4-[3-cyano-2-oxo-7-(1H-pyrazol-4-yl)-5,6-dihydro-1H-benzo[h]quinolin-4-yl]benzoic 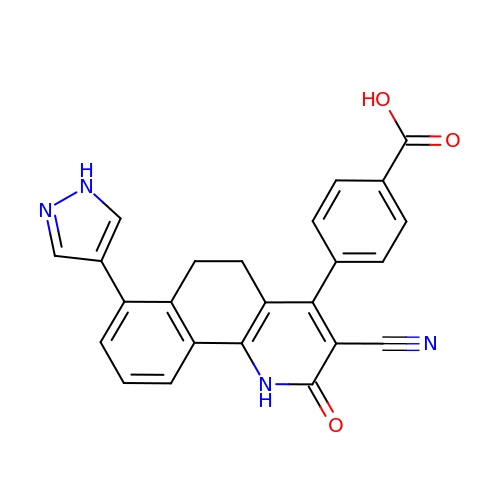acid | C24 H16 N4 O3 | STALUGJGAYBZIU-UHFFFAOYSA-N>[2x]MVYSKEIVREWLDEVAERAKDYPEWVDVFERCYTDTLDNTVEILEDGSTFVLTGDIPAMWLRDSTAQLRPYLHVAKRDALLRQTIAGLVKRQMTLVLKDPYANSFNIEENWKGHHETDHTDLNGWIWERKYEVDSLCYPLQLAYLLWKETGETSQFD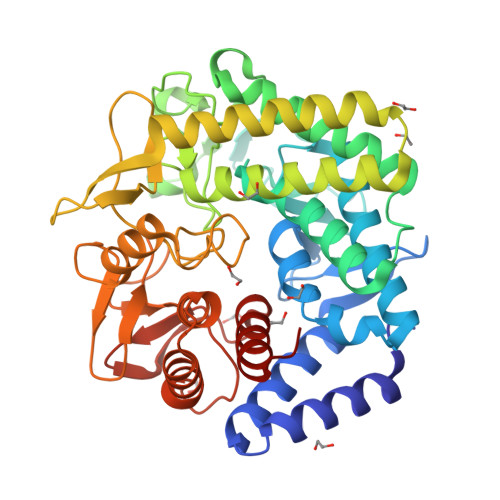EIFVAATKEILHLWTVEQDHKNSPYRFVRDTDRKEDTLVNDGFGPDFAVTGMTWSAFRPSDDCCQYSYLIPSNMFAVVVLGYVQEIFAALNLADSQSVIADAKRLQDEIQEGIKNYAYTTNSKGEKIYAFEVDGLGNASIMDDPNVPSLLAAPYLGYCSVDDEVYQATRRTILSSENPYFYQGEYASGLGSSHTFYRYIWPIALSIQGLTTRDKAEKKFLLDQLVACDGGTGVMHESFHVDDPTLYSREWFSWANMMFCELVLDYLDIR> MSADNGLIIGIDLGTTNSCVSVMEGGRPVVLENPEGKRTTPSIVSYKNNEIIVGDAAKRQMVTNPNTIVSIKRLMGTSNKVKVQNADGTTKELSPEQVSAQILSYLKDFAEKKIGKKISRAVITVPAYFNDAERNATKTAGKIAGLNVER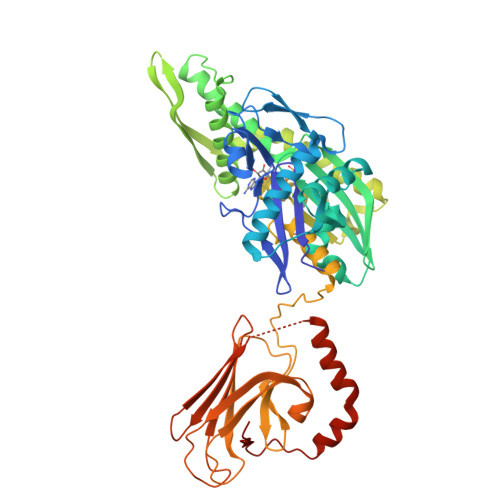IINEPTAAALAYGIDKASREMKVLVYDLGGGTFDVSLLDIAEGTFEVLATAGDNRLGGDDWDNKIIEYISAYIAKEHQGLNLSKDKMAMQRLKEAAERAKIELSAQLETIISLPFLTVTQKGPVNVELKLTRAKFEELTKPLLERTRNPISDVIKEAKIKPEEINEILLVGGSTRMPAVQKLVESMVPGKKPNRSINPDEVVAIGAAIQGGVLRGDVKDVLLLDVTPLTLSIETLGGVATPLIKRNTTIPVSKSQIFSTAQDNQESVDVVVCQGERPMSRDNKSLGRFNLGGIQPAPKGKPQIEITFSLDANGILNVKAKDLTTQKENSITISDNGNLSEEEIQKMIRDAEANKERDNIIRERIELRNEGELEHHHHHH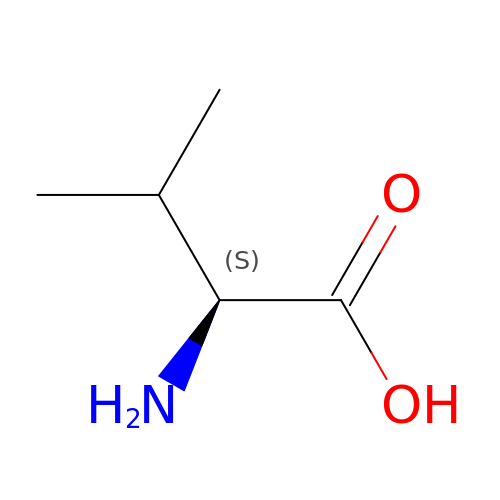VALINE | C5 H11 N O2 | KZSNJWFQEVHDMF-BYPYZUCNSA-N>[2x]MTENFFGKTLAARPVEAIPGML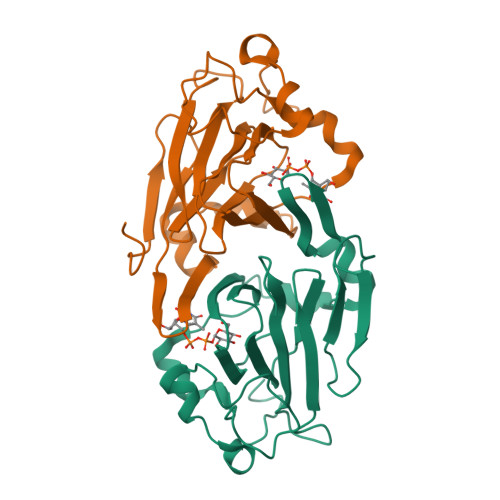EFDIPVHGDNRGWFKENFQKEKMLPLGFPESFFAEGKLQNNVSFSRKNVLRGLHAEPWDKYISVADGGKVLGTWVDLREGETFGNTYQTVIDASKSIFVPRGVANGFQVLSDFVAYSYLVNDYWALELKPKYAFVNYADPSLDIKWENLEEAEVSEADENHPFLKDVKPLRKEDL>MAHHHHHHMSSAGRLQGKVALVTGAGCIGPGWGNGRAIAVRFAEEGAHVIAVDRDLASMDATLELVRAAGGSVTPCLCDVTDSASVERLVADSVARCGRVDILVNNVGAPSPGGPVALDEAQWAMQLELNLTTAFLMCKYVLPVMEQQGGGAIVNIASTSGIRWTGAAQVGYAAAKAGMIQMGRVVAVEYAAKNVRVNSVVPGLLHTPMVDTKIAHNQAGGDVELLLRKRQARIPMPFMGDGRDTANAALFLAS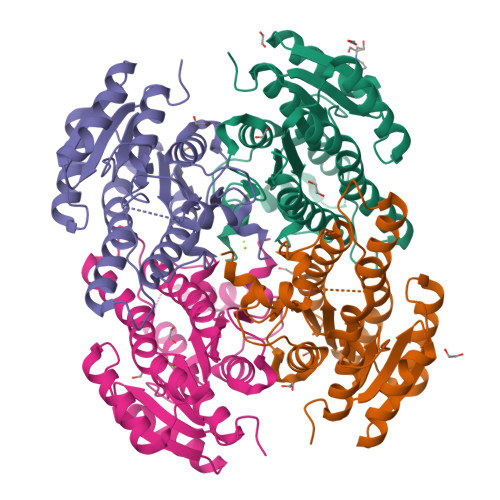DEARFVTGTEIVVDGGMSARCD[4x]>AFGITTSSSAYVIDTNAPNQLKFTVSRSSCDITSIIHYGTELQYSSQGSHIGSGLGSATVTATQSGDYIKVTCVTDTLTQYMVVHNGDPIIHMATYITAEPSIGELRFIARLNSDLLPNEEPFGDVSTTADGTAIEGSDVFLVGSETRSAFYSSERFIDDQRHCIAGDAHRVCMILNQYESSSGGPFHRDINSNNGGSYNALYWYMNSGHVQTESYRMGLHGPYSMYFSRSGTPSTSIDTSFFADLDIKGYVAASGRGKVAGTASGADS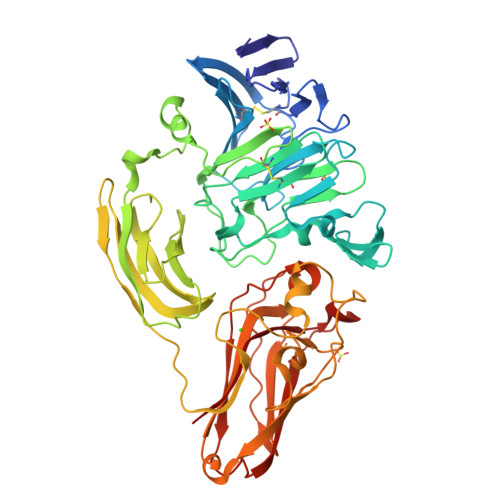SMDWVVHWYNDAAQYWTYTSSSGSFTSPAMKPGTYTMVYYQGEYAVATSSVTVSAGSTTTKNISGSVKTGTTIFKIGEWDGQPTGFRNAANQLRMHPSDSRMSSWGPLTYTVGSSALTDFPMAVFKSVNNPVTIKFTATSAQTGAATLRIGTTLSFAGGRPQATINSYTGSAPAAPTNLDSRGVTRGAYRGLGEVYDVSIPSGTIVAGTNTITINVISGSSGDTYLSPNFIFDCVELFQ[2x]>GSEELLDLFNRQVTQEFTASQVYLSASIWFDQNDWEGMAAYMLAQSAEEREHGLGFVDFANKRNIPIELQAVPAPVSCAEWSSPEDVWQSILELEQANTRSLLNLAEAASTCHDF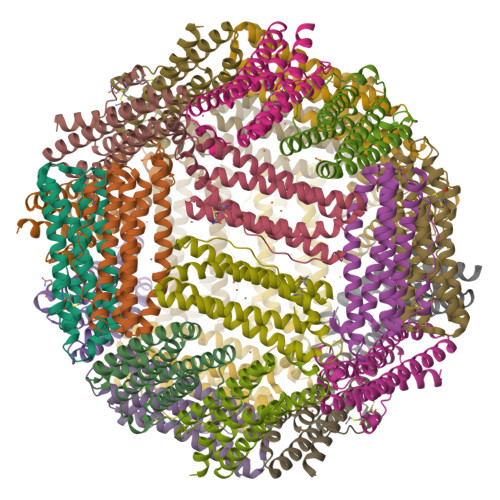AVMAFLNPFHLQQVNEEDKIGSILAKVTDENRTPGLLRSLDVVSFLGPCLFRSV[8x]>[6x]QLTPTFYDNSCPNVSNIVRDTIVNELRSDPRIAASILRLHFHDCFVNGCDASILLD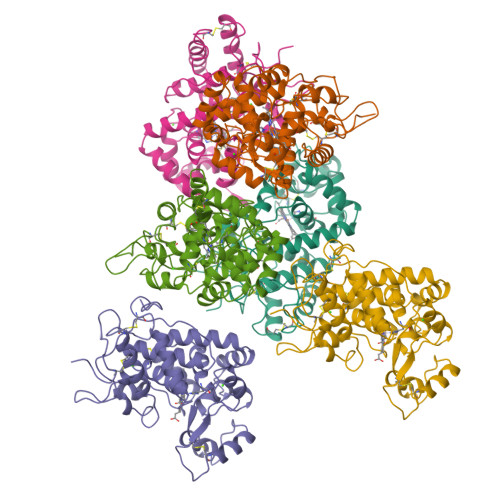NTTSFRTEKDAFGNANSARGFPVIDRMKAAVESACPRTVSCADLLTIAAQQSVTLAGGPSWRVPLGRRDSLQAFLDLANANLPAPFFTLPQLKDSFRNVGLNRSSDLVALSGGHTFGKNQCRFIMDRLYNFSNTGLPDPTLNTTYLQTLRGLCPLNGNLSALVDFDLRTPTIFDNKYYVNLEEQKGLIQSDQELFSSPNATDTIPLVRSFANSTQTFFNAFVEAMDRMGNITPLTGTQGQIRLNCRVVNS The anaerobic, Ni-dependent CODH has a homodimeric structure containing a total of five metalloclusters, called the B-, C-, and D-clusters. The C-cluster is the site of CO/CO2 interconversion and is composed of a [Ni-3Fe-4S] cubane connected through a linking sulfide (SL) to a unique iron site (Feu). Here, we report the crystal structure of the CODH from Desulfovibrio vulgaris (DvCODH), which reveals a surprising and unprecedented conformational rearrangement of metal ions in the C-cluster and provides the first visualization of the cluster in an oxidized state. The overall fold and cluster placement of DvCODH is highly similar to other structurally characterized CODHs.

One of the more noteworthy aspects of the oxidized C-cluster is that cluster ligation involves one residue (Cys301) that is strictly conserved in CODHs but is not a ligand to the canonical C-cluster. To probe the effect of Cys301 in DvCODH, a DvCODH(C301S) variant was produced and characterized. Similar to what was observed with MtCODH/ACS, DvCODH(C301S) is inactive and does not contain Ni, as assessed by CO oxidation activity assays and inductively coupled plasma optical emission spectroscopy (ICP-OES), respectively. Unlike wild-type DvCODH, DvCODH(C301S) cannot be activated by Ni under reducing conditions, analogous to what has been observed previously for DvCODH samples grown in the absence of the C-cluster maturation factor CooC. To investigate the architecture of a non-activatable C-cluster, we determined the crystal structure of DvCODH(C301S) to 2.0 Å resolution and discovered an intact [3Fe-4S] C-cluster core with an Feu ion that adopts alternative conformations. Approximately 70% of Feu is in its canonical position coordinated by His266 and Cys302, whereas approximately 30% is in the Ni-cubane site. Thus, in the absence of the non-canonical Feu-ligand Cys301, the cluster cannot be activated by Ni and Feu appears to be free to occupy multiple sites. Taken together, these data suggest that the novel structure of the C-cluster that we observe here, with Feu coordinated by Cys301, is relevant to processes beyond oxidation, specifically Ni incorporation.

>MWSHPAVRKSSSKTIRSRSIWDDAHAMLEKAKAEGISTVWDRAAEQTPACKFCELGTTCRNCIMGPCRIANRKDGKMRLGVCGADADVIVARNFGRFIAGGAAGHSDHGRDLIETLEAVAEGKAPGYTIRDVAKLRRIAAELGVADAATRPAHDVAADLVTICYNDFGSRRNALAFLARAPQVRRDLWQRLGMTPRGVDREIAEMMHRTHMGCDNDHTSLLVHAARTALADGWGGSMIGTELSDILFGTPRPRQSTVNLGVLRKDAVNILVHGHNPVVSEMILAATREPAVRQAAQDAGAADINVAGLSCTGNELLMRQGIPMAGNHLMTELAIVTGAADAIVADYQCIMPSLVQIAACYHTRFVTTSPKGRFTGATHVEVHPHNAQERCREIVMLAIDAYTRRDPARVDIPSQPVSIMSGFSNEAILEALGGTPKPLIDAVVAGQIRGFVGIVGCNNPKIRQDSANVTLTRELIRRDIMVLATGCVTTAAGKAGLLVPEAASKAGEGLAAVCRSLGVPPVLHMGSCVDNSRILQLCALLATTLGVDISDLPVGASSPEWYSEKAAAIAMYAVASGIPTHLGLPPNILGSENVTAMALHGLQDVVGAAFMVEPDPVKAADMLEAHIVARRARLGLTS[4x]> MDSLDQCIVNACKNSWDKSYLAGTPNKDNCSGFVQSVAAELGVPMPRGNANAMVDGLEQSWTKLASGAEAAQKAAQGFLVIAGLKGRTYGHVAVVISGPLYRQKY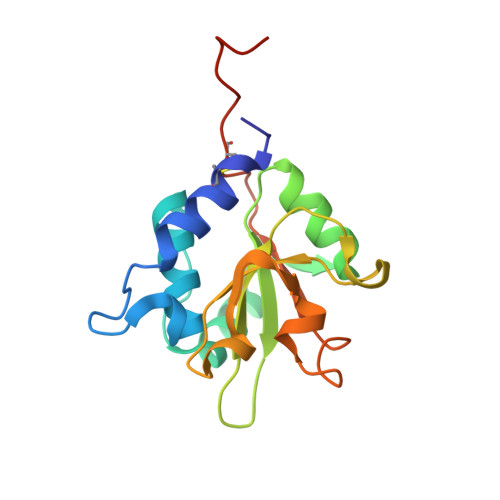PMCWCGSIAGAVGQSQGLKSVGQVWNRTDRDRLNYYVYSLASCSLPRASLEHHHHHH> MPTLLRVYIDGPHGMGKTTTTQLLVALGSRDDIVYVPEPMTYWRVLGASETIANIYTTQHRLDQGEISAGDAAVVMTSAQITMGMPYAVTDAVLAPHIGGEAGSSHAPPPALTLIFDRHPIAALLCYPAARYLMGSMTPQAVLAFVA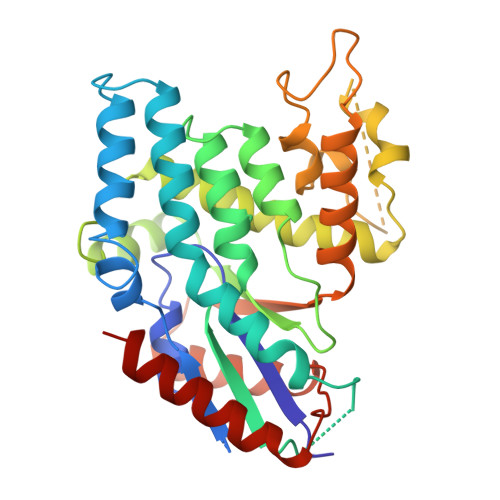LIPPTLPGTNIVLGALPEDRHIDRLAKRQRPGERLDLAMLAAIRRVYGLLANTVRYLQCGGSWREDWGQLSGTAVPPQGAEPQSNAGARPHIGDTLFTLFRAPELLAPNGDLYNVFAWALDVLAKRLRSMHVFILDYDQSPAGCRDALLQLTSGMVQTHVTTPGSIPTICDLARTFAREMGEAN> MERAEILGVGTELLYGETLDTNTAEIARSLKPYALKVERTLRVADEVAPLAREVEEAFARARLVVLSGGLGPTPDDVTREAVALALGEPLELDEAVLGEIEAFFRARGRAMPEANRKQAMRIPSATWLKNPRGTAPGWWVRKGGKDLVLLPGPPPEWRPMWQEVLPRLGLPRRPYAERVLKTWGIGESEIVERLGPLFVREEEEEVGTYPKVHGVEVVVRGREDRVAELAERIKKKLLKEVWGEGEMTLAEAVKRRMEREGATLSTMESLTGGLLGAEITRVPGASRFYLGGVVSYSVGAKARFGVPQDLLSRTVSAETARAMAEAARSLFGSTYALATTGVAGPDPLEGEPPGTVYVALAGPTGAEVRRYRFPGDRETVRLRSVYAALALLVT;> MERAEILGVGTELLYGETLDTNTAEIARSLKPYALKVERTLRVADEVAPLAREVEEAFARARLVVLSGGLGPTPDDVTREAVALALGEPLELDEAVLGEIEAFFRARGRAMPEANRKQ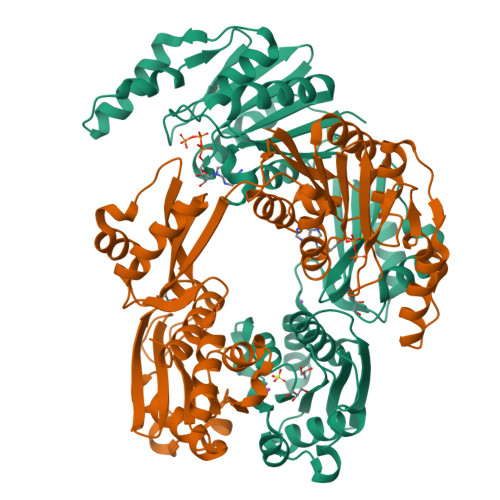AMRIPSATWLKNPRGTAPGWWVRKGGKDLVLLPGPPPEWRPMWQEVLPRLGLPRRPYAERVLKTWGIGESEIVERLGPLFVREEEVEVGTYPKVHGVEVVVRGREDRVAELAERIKKKLLKEVWGEGEMTLAEAVKRRMEREGATLSTMESLTGGLLGAEITRVPGASRFYLGGVVSYSVGAKARFGVPQDLLSRTVSAETARAMAEAARSLFGSTYALATTGVAGPDPLEGEPPGTVYVALAGPTGAEVRRYRFPGDRETVRLRSVYAALALLVT6-{[(1R,2S)-2-aminocyclohexyl]amino}-5-cyano-2-[(3-methylphenyl)amino]pyridine-3-carboxamide | C20 H24 N6 O | 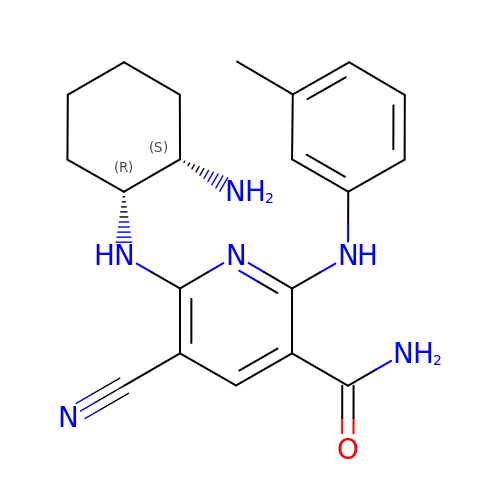XAMCCSYNPOEISO-DLBZAZTESA-N> MAHHHHHHMFDIQEIRSQFPILQEKVNGKDLVYLDNAATSQKPKMVLDAINNYYEHYNANVHRGIHTLSQVATEMMEDARKKVQRFINAKHDYEVLFTKGTTEGINLV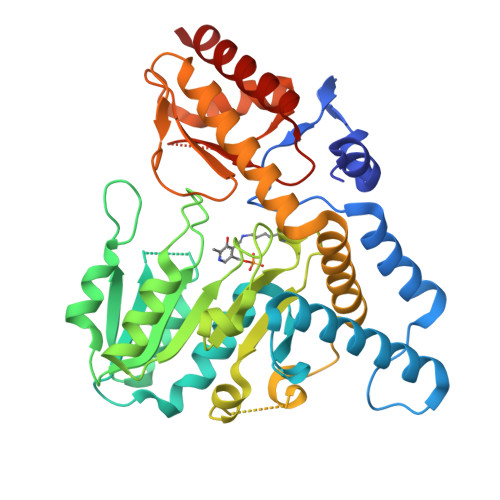AYAMTDLIKKDDEIIISYLEHHSNIVPWQMLCQRTGAKLRVIPMNEDGTLQIDVLDEWLSEKTKLVSVNQVSNALGIVNPIDEIIRKVRAKSNAFIFIDGAQAAPHFEIDVQTMDCDFFAFSGHKMYGPTGTGILYGKASVLEQLNPFHGGGEMIDHCTFEKTTYAGLPFRFEAGTPNIAGNIAIGTAVDFMEKVGRSNIAAHEHALLEYAQRKLLEIEGLKVYGEKANRAGVVSFNLSGIGIASDVGMILDKLGIAVRTGHHCTQPIMEYFGVAGTVRASFAVYNTFEEIDILTEGVKKAQKMLA> GPMP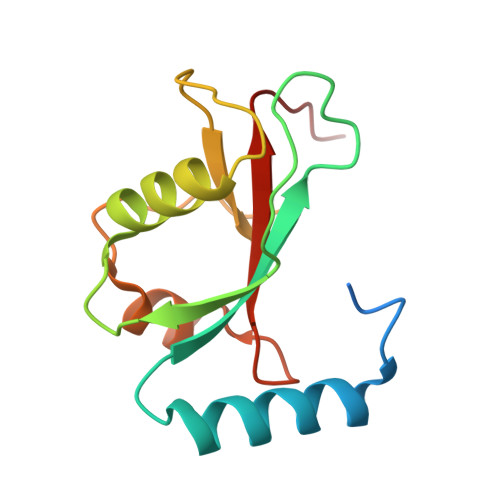PPQKIPSVRPFKQRKSLAIRQEEVAGIRAKFPNKIPVVVERYPRETFLPPLDKTKFLVPQELTMTQFLSIIRSRMVLRATEAFYLLVNNKSLVSMSATMAEIYRDYKDEDGFVYMTYASQETFG> MHHHHHHMAQVINTNSLSLLTQNNLNKSQSALGTAIERLSSGLRINSAKDDAAGQAIANRFTANIKGLTQASRNANDGISIAQTTEGALNEINNNLQRVRELAVQSANSTNSQSDLDSIQAEITQRLNEIDRVSGQTQFNGVKVLAQDNTLTIQVGANDGETIDIDLKQINSQTLGLDTLNVQQKYKVSDTAATVTGYADTTIALDNSTFKASATGLGGTDQKIDGDLKFDDTTGKYYAKVTVTGGTGKDGYYEVSVDKTNGEVTLAGGATSPLTGGLPATATEDVKNVQVANADLTEAKAALTAAGVTGTASVVKMSYTDNNGKTIDGGLAVKVGDDYYSATQNKDGSISINTT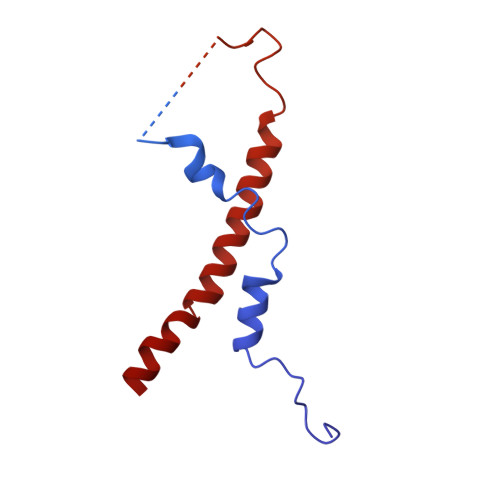KYTADDGTSKTALNKLGGADGKTEVVSIGGKTYAASKAEGHNFKAQPDLAEAAATTTENPLQKIDAALAQVDTLRSDLGAVQNRFNSAITNLGNTVNNLTSARSRIEDSDYATEVSNMSRAQILQQAGTSVLAQANQVPQNVLSLLR> MVAASEGNVVIEVDMANGWRGNASGSTSHSGITYSADGVTFAALG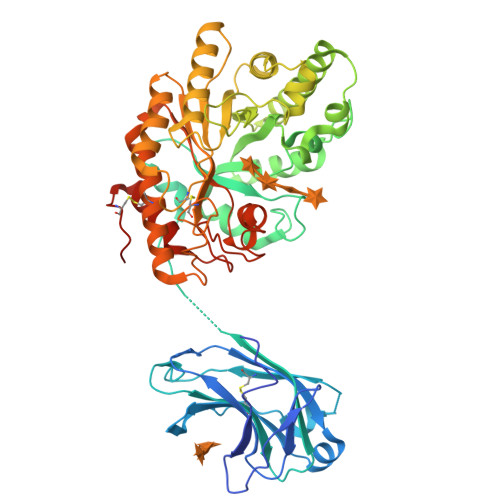DGVGAVFDIARPTTLEDAVIAMVVNVSAEFKASEANLQIFAQLKEDWSKGEWDCLAASSELTADTDLTLTCTIDEDDDKFNQTARDVQVGIQAKGTPAGTITIKSVTITLAQEAYSANVDHLRDLAPSDFPIGVAVSNTDSATYNLLTNSREQAVVKKHFNHLTAGNIMKMSYMQPTEGNFNFTNADAFVDWATENNMTVHGHALVWHSDYQVPNFMKNWAGSAEDFLAALDTHITTIVDHYEAKGNLVSWDVVNAAIDDNSPANFRTTDSAFYVKSGNSSVYIERAFQTARAADPAVILYYNDYNIEQNNAKTTKMVDMVKDFQARSIPIDGVGFQMHVCMNYPSIANISAAMKKVVDLGLLVKITELDVAVNQPHCDAYPANKINPLTEAAQLAQKKRYCDVVKAYLDTVPVNQRGGISVWGTTDANTWLDGLYREQFEDEKISWPLLFDNNYNDKPALRGFADALIGTQCTNTHELHHHHHH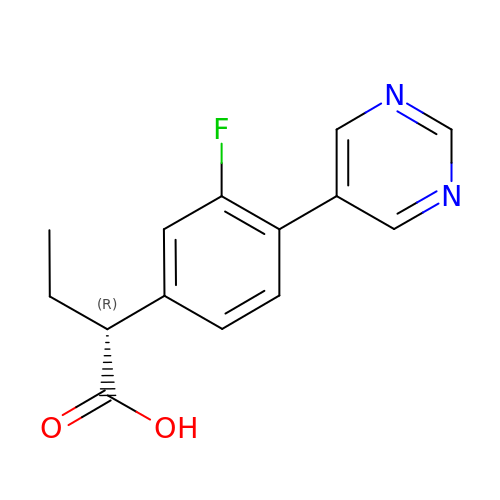(2~{R})-2-(3-fluoranyl-4-pyrimidin-5-yl-phenyl)butanoic acid | C14 H13 F N2 O2 | LKTIRPQROJRUNF-LLVKDONJSA-N> ADSGEGDFLAEGGGVRGPRVVERHQSACKDSDWPFCSDEDWNYKCPSGCRMKGLIDEVNQDFTNRINKLKNSLFEYQKNNKDSHSLTTNIMEILRGDFSSANNRDNTYNRVSEDLRSRIEVLKRKVIEKVQHIQLLQKNVRAQLVDMKRLEVDIDIKIRSCRGSCS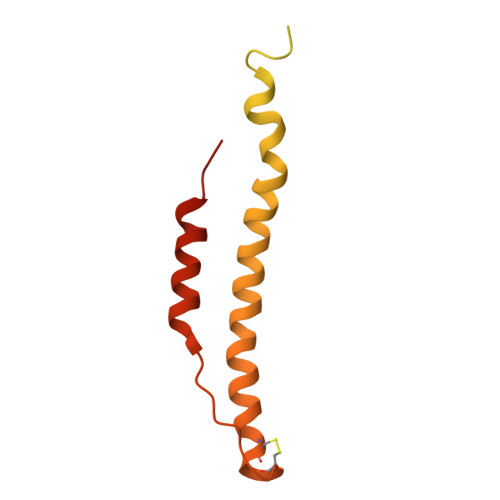RALAREVDLKDYEDQQKQLEQVIAKDLLPSR>[3x]SLKPLTLLMTSSTSFSETINQWADILKTTDMEKFSFDSNPINLLELVKQFNLYVDELAITCEANNVWAKERIDSTPNLFALYDNSGGEAIHGHAFVPYYKESIVLRRLFTVDPNTFNLSRFAAFEGPCQLYCKEHKDSAWVKIQTLLTLGNGIINTLKIIKQAQAFGIDE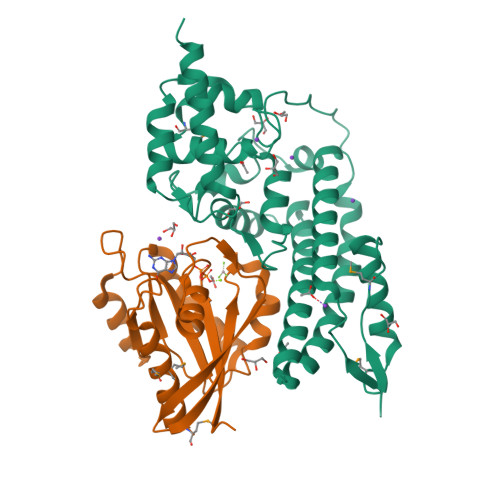AVTENLKALKEQFIAFQLAEADIKESLKAPSFAEPLPNKESEFFYPIDEKALAKMNGYQLATICLEELNSPKPSPLIERILSNKKFWKRINSAFESGVFKGRTDDPAGKIAKIREWHQLLQISGKKTAG;>MGHHHHHHGSMNPEYDYLFKLLLIGDSGVGKSCLLLRFADDTYTESYISTIGVDFKIRTIELDGKTIKLQIWDTAGQERFRTITSSYYRGAHGIIVVYDVTDQESFNNVKQWLQEIDRYASENVNKLLVGNKCDLTTKKVVDYTTAKEFADSLGIPFLETSAKNATNVEQSFMTMAAEIKKRMG[3x]> GHMASMLYLLDKSDYPKVKHLVRTKEEKSDVPLNAVINGTNVGNIYVDDPDHPKAALVDAVGTTCFLIGDASSPVFGEHLKDCIENQLKDQCLESGGSYFIATLFDKEWEKVLENAISHREYEPDYEFYHEFDKDKFNKVKSNYRSLTNEYTIKRMDKELIQNDSDDTLRSCLSDFWDSIDDFLTKG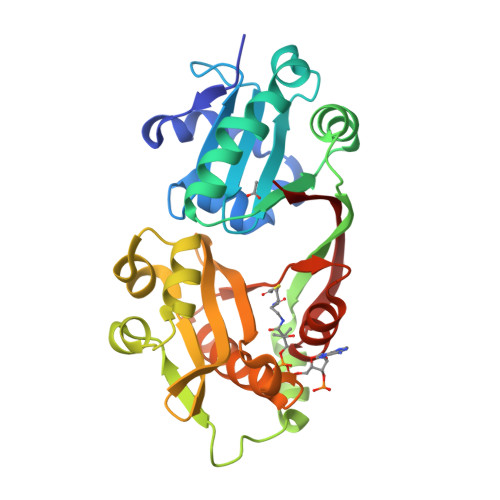VGFCVIKDEQVISSCFTCYVDGNNHEISVETYDEEEQNKGLATKACEVYLEYCIENGITPHWSTFETNVESVNLASKLGFEYRFKLKTYEFEY>[2x]MEELTYRLFMVATVGMLAGTVFLLASSREVKPEHRRGVYISALVCGIAWYHYQKMGASWESGSYDTGLRYVD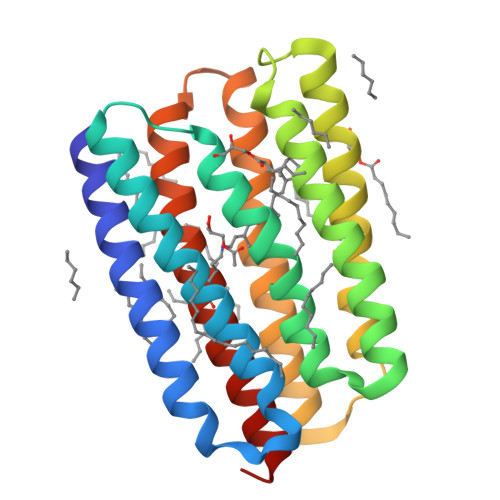WVLTVPLMFVEVLAVTRKGAAYNEAVRNWGIAATVMIGAGYYGETSAAGSNEYWTGFVIAMATYVWLMRNLQAEGEGLKGDQAVAFENIKNLILVGWIIYPLGYIAPVVGDFDAIREVLYTIADIINKVGLGVLVLQMARVQSGEKVS>GQIQISKHVKDVGLPSIHTPTKTKLQPSVFYDIFPGSKEPAVLTEKDPRLKVDFDSALFSKYKGNTECSLNEHIQVAVAHYSAQLATLDIDPQPIAMEDSVFGMDGLEALDLNTSAGYPYVTLGIKKKDLINNKTKDISKLKLALDKYDVDLPMITFLKDELRKKDKIAAGKTRVIEASSINDTILFRTVYGNLFSKFHLNPGVVTGCAVGCDPETFWSKIPLMLDGDCIMAFDYTNYDGSIHPIWFKALGMVLDNLSFNPTLINRLCNSKHIFKSTYYEVEGGVPSGCSGTSIFNSMINNIIIRTLVLDAYKHIDLDKLKIIAYGDDVIFSYKYKLDMEAIAKEGQKYGLTITPADKSSEFKELDYGNVTFLKRGFRQDDKYKFLIHPTFPVEEIYESIRWTKKPSQMQEHVLSLCHLMWHNGPEIYKDFETKIRSVSAGRALYIPPYELLRHEWYEKF[4x]

The replication of positive-strand RNA viruses relies on virally encoded RNA-dependent RNA polymerases (RdRPs) that are capable of rapid and processive synthesis of the 7–14 kilobase viral genomes. To examine this in further detail and to validate the polymerase–RNA interactions seen in the initial poliovirus EC structures, we here present nine new coxsackievirus, rhinovirus, and poliovirus elongation complex structures at resolutions ranging from 2.1 to 2.9 Å. All the complexes feature an upstream RNA duplex that is pinched between the pinky finger and thumb domains such that the RNA exit channel is opened by ≈4 Å as compared to the polymerase alone structures. All of the complexes show the open conformation for the active site wherein the β-strands of motifs A and C are not hydrogen bonded together to fully form the RMM-fold that is commonly utilized by polymerase active sites.

Using the r1 RNA used to crystallize and solve the initial PV polymerase EC structure (i.e. PV_r1), we were able to also crystallize the RV polymerase EC (RV_r1). The RV EC structure retained the coaxially stacked EC pairs seen with the original poliovirus structure, but note that the two RV EC pairs are in a very different spatial arrangement than previously observed. Note that the NCS pairs in the RV_r1 structure are in different dumbbell pairs while those of the other structures are within each dumbbell pair. The RV_r1 EC is the only structure where we observe significant contacts involving the downstream template duplex, but these appear to be non-specific interactions with other polymerase molecules in the lattice and not a biologically relevant interface. The contact stabilizes the orientation of the RNA helix, resulting in strong electron density into which we could build the entire 6-base pair hairpin and tetra-loop sequence. In contrast, there are no indications of conserved protein-RNA interactions further downstream of the +2 position; all the RNAs tested included a downstream duplex, but only in the RV_r1 structure did we observe sufficient electron density to model the full downstream RNA hairpin due to the fact that the RV_r1 helix is held in place via non-specific interactions with other polymerases in the crystal lattice.PCNA encircling duplex DNA is quite stable and is removed from DNA by the dedicated clamp unloader Elg1-RFC. The three alternative RFC-like complexes are formed by replacement of the large subunit, Rfc1 of RFC, with Rad24, Ctf18, or Elg1 (16). Specifically, Elg1 contains two external loops that block opening of the Elg1-RFC complex for DNA binding, and an “Elg1 plug” domain that fills the central DNA binding chamber, thereby reinforcing the exclusive PCNA unloading activity of Elg1-RFC. In all three Elg1-RFC structures, we found five bound nucleotides: four ATPγS in Rfc2, Rfc3, Rfc4, and Elg1, and one ADP in Rfc5 (top right).

By leveraging state-of-the-art cryo–electron microscopy (cryo-EM), we find that the architecture of Elg1-RFC is specifically suited to the unloading of PCNA. This report documents Elg1-RFC alone and Elg1-RFC bound to a closed PCNA clamp and to a cracked PCNA clamp at 3.2-, 3.3-, and 3.7-Å resolution, respectively. Because clamp unloading starts with PCNA encircling dsDNA, we propose that the three structures that we have determined represent (i) Elg1-RFC alone before it encounters a PCNA, (ii) Elg1-RFC that has taken the PCNA off DNA with the clamp being incompletely closed (i.e., cracked PCNA), and (iii) Elg1-RFC bound to the closed PCNA after PCNA is taken off DNA (Elg1-RFC–closed PCNA), respectively. The shared Elg1-RFC among the three structures is highly similar with a root mean square deviation between main chain Cα atoms in the range of 0.5 to 0.6 Å. The first loop (LL1) is 57-residue long between Arg184 and Thr240, preceding the AAA+ domain and emanating from between the collar domains of Rfc2 and Rfc3 and wraps around the collar domains of Rfc3 and Rfc4, whereby the C-terminal half (LL1C) cross-links the A-gate (top right). The LL2 loop is 25-residue long (Cys511 to Ser535) and corresponds to the “alternative linker” loop in Rfc1 of RFC. Together, the Elg1-RFC A-gate is locked by the LL1 and LL2 loops into a closed and static state, which is unable to open to bind DNA. The Rfc1 collar domain contains five α helices, but two of the five α helices in the Elg1 collar domain have descended to form the Elg1 plug, with only three α helices remaining at the top collar tier. The Elg1 plug interacts with and is extensively stabilized by all Elg1-RFC subunits except for Rfc2. Given the extensive interactions, the Elg1 plug is likely immobile during the PCNA unloading process. The structure of Elg1-RFC indicates that it cannot bind dsDNA in the central chamber or the shoulder binding site.

> MKRHVSLSDILTGNKRKVRRQDALQITIDDENDTESGTFDARTAKHDDSSVIFLNHSVVKPIEAVSTNHKSAKEFLMTKRTKEKCDDDDDDLIVISDKSPKSETNCSKIALSQEHEDDISIISTSRIKSSLLNERASKIKNFLKHETTDTFKRLNSISKLNEIEPPLPLHQSIFPVGDKELSDRSVDIPLPFRTIPPLNHNFLPSDYESLKDKNSASCIPVRYQAPVLLGTNIKRNTTLTWPQLFKPVTLKQVLIEPKLKLRIKNWIETSFHTLEKPTLRNRLLNRINPNKQQGSGDELANFIVPDLEEDENLRPDFYRNGEANSSLSEFVPLMILHGNSIGKKTLIQTIMREIAGDDNSYQIYEVNSNMNRSKKDLLDILLDFTTTHYVKDSSKRKSDYGLVLFNDVDVLFKEHDRGYWAMISKLCEFSRRPLVLTCKDLSLVPSELIALASEQNSLFHTKKISTSTVYAFLTKYLKSLEIEVCDDWLRDVVKQNNADIRKCLMHLQFWCVDTEADLISSKNRLPVLTSTLGSSVKDISQLTDLLSINDVIGQATLNRSMVRQEIDSTTMTPEKVNTFQDQNLDDEMKLKFDYVIDYKLHLNDPNRQPLLPFELNIYQHIQEQLEARYSYVREANHRLDNEYLVNRFKKMTESTLNFLASRIPKYDHLQSARRTRNSKKISDILNQFKGIYNDETLNENAEIDLLSATTQQIKAEINPFVFEIAKSDANVKNENKQIFELHSENVSERRYKDLVYQLSQEGVLKNVWFNADPSIVVRKWEHLHSGFSKNK;> MSKTLSLQLPWVEKYRPQVLSDIVGNKETIDRLQQIAKDGNMPHMIISGMPGIGKTTSVHCLAHELLGRSYADGVLELNASDDRGIDVVRNQIKHFAQKKLHLPPGKHKIVILDEADSMTAGAQQALRRTMELYSNSTRFAFACNQSNKIIEPLQSRCAILRYSKLSDEDVLKRLLQIIKLEDVKYTNDGLEAIIFTAEGDMRQAINNLQSTVAGHGLVNADNVFKIVDSPHPLIVKKMLLASNLEDSIQILRTDLWKKGYSSIDIVTTSFRVTKNLAQVKESVRLEMIKEIGLTHMRILEGVGTYLQLASMLAKIHKLNNKA;> MSTSTEKRSKENLPWVEKYRPETLDEVYGQNEVITTVRKFVDEGKLPHLLFYGPPGTGKTSTIVALAREIYGKNYSNMVLELNASDDRGIDVVRNQIKDFASTRQIFSKGFKLIILDEADAMTNAAQNALRRVIERYTKNTRFCVLANYAHKLTPALLSRCTRFRFQPLPQEAIERRIANVLVHEKLKLSPNAEKALIELSNGDMRRVLNVLQSCKATLDNPDEDEISDDVIYECCGAPRPSDLKAVLKSILEDDWGTAHYTLNKVRSAKGLALIDLIEGIVKILEDYELQNEETRVHLLTKLADIEYSISKGGNDQIQGSAVIGAIKASFENETV;> MFEGFGPNKKRKISKLAAEQSLAQQPWVEKYRPKNLDEVTAQDHAVTVLKKTLKSANLPHMLFYGPPGTGKTSTILALTKELYGPDLMKSRILELNASDERGISIVREKVKNFARLTVSKPSKHDLENYPCPPYKIIILDEADSMTADAQSALRRTMETYSGVTRFCLICNYVTRIIDPLASRCSKFRFKALDASNAIDRLRFISEQENVKCDDGVLERILDISAGDLRRGITLLQSASKGAQYLGDGKNITSTQVEELAGVVPHDILIEIVEKVKSGDFDEIKKYVNTFMKSGWSAASVVNQLHEYYITNDNFDTNFKNQISWLLFTTDSRLNNGTNEHIQLLNLLVKISQL;> MSLWVDKYRPKSLNALSHNEELTNFLKSLSDQPRDLPHLLLYGPNGTGKKTRCMALLESIFGPGVYRLKIDVRQFVTASNRKLELNVVSSPYHLEITPSDMGNNDRIVIQELLKEVAQMEQVDFQDSKDGLAHRYKCVIINEANSLTKDAQAALRRTMEKYSKNIRLIMVCDSMSPIIAPIKSRCLLIRCPAPSDSEISTILSDVVTNERIQLETKDILKRIAQASNGNLRVSLLMLESMALNNELALKSSSPIIKPDWIIVIHKLTRKIVKERSVNSLIECRAVLYDLLAHCIPANIILKELTFSLLDVETLNTTNKSSIIEYSSVFDERLSLGNKAIFHLEGFIAKVMCCLD>MAHHHHHHMLYPLVK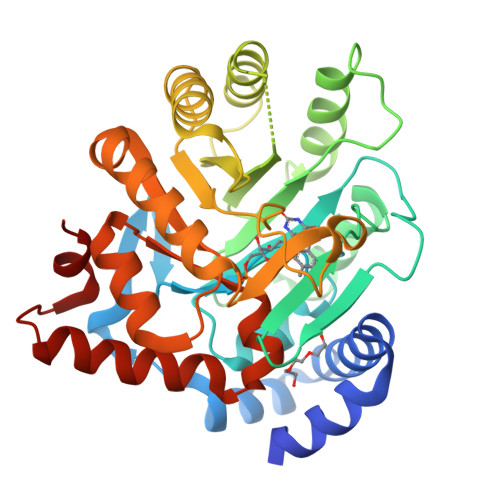KYLFSLDAEDAHEKVCKILRTLSKSSFLCSLIHSQWGYKNPKLENEILGLNFPNPLGLAAGFDKNASMLRALIAFGFGYLEAGTLTNEAQVGNERPRLFRHIEEESLQNAMGFNNYGAVLGARSFNRFAPYKTPIGINLGKNKHIEQAHALEDYKAVLNQCLNIGDYYTFNLSSPNTPNLRDLQNKAFVNELFCMAKEMTHKPLFLKIAPDLEIDDMLEIVNSAIEAGAHGIIATNTTIDKSLVFAPKEMGGLSGKCLTKKSREVFKELAKAFFNKSVLVSVGGISDAKEAYERIKMGASLLQIYSAFIYNGPNLCQNILKDLVKLLQKDGFLSVKEAIGADLR[2x]> MSDSSQLHKVAQRANRMLNVLTEQVQLQKDELHANEFYQVYAKAALAKLPLLTRADVDYAVSEMEEKGYVFDKRPAGSSMKYAMSIQNIIDIYEHRGTPKYRDRYSEAYVIFISNLKGGVSQTTSTVSLAHAMRAHPHLLMEDLRILVIDLDPQSSATMFLSHKHSIGIVNATSAQAMLQNVSREELLEEFIVPSVVPGVDVMPASIDDAFIASDWRELC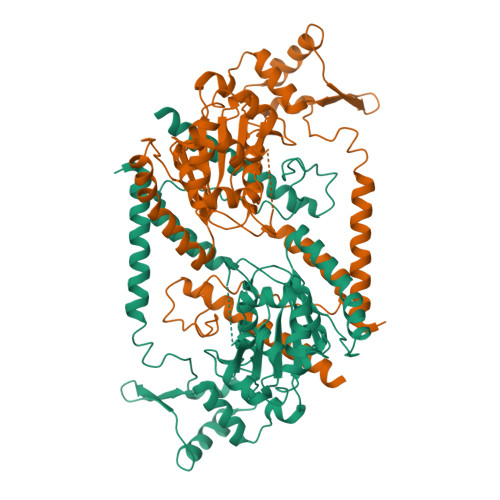NEHLPGQNIHAVLKENVIDKLKSDYDFILVDSGPHLDAFLKNALASANILFTPLPPATVDFHSSLKYVARLPELVKLISDEGCECQLATNIGFMSKLSNKADHKYCHSLAKEVFGGDMLDVFLPRLDGFERCGESFDTVISANPATYVGSADALKNARIAAEDFAKAVFDRIEFIRSN>[4x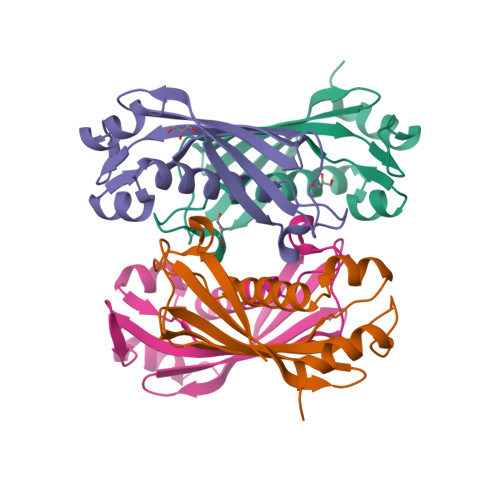]MESVTRIKVRYAETDQMGVVHHSVYAVYLEAARVDFLERAGLPYHRVEARGVFFPVVELGLTFRAPARFGEVVEVRTRLAELSSRALLFRYRVEREGVLLAEGFTRHLCQVGERAARIPEDIYRALSVLHLK> MKKEKIDLFYGALLADIGKVIQRATGERKKHALVGADWFDEIADNQVISDQIRYHMANYQSDKLGNDHLAYITYIADNIASGVDRRQSNEESDEDTSAKIWDTYTNQADIFNVFGAQTDKRYFKPTVLNLKSKPNFASATYEPFSKGDYAAIATRIKNELAEFEFNQVQIDSLLNLFEATLSFVPSSTNTKEIADISLADHSRLTAAFALAIYDYLEDKGRHNYKEDLFTKVSAFYEEEAFLLASFDLSGIQDFIYNINIATNGAAKQLKARSLYLDFMSEYIADSLLDKLGLNRANMLYVGGGHAYF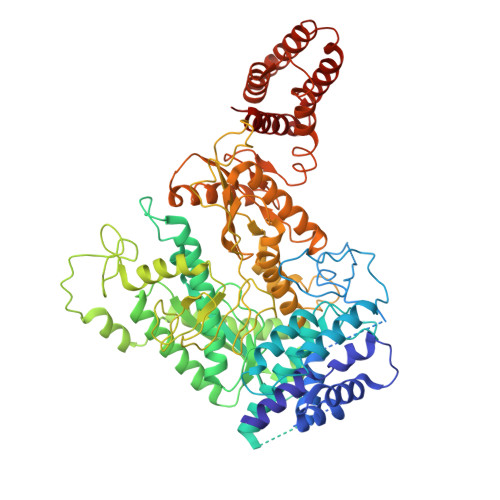VLANTEKTVETLVQFEKDFNQFLLANFQTRLYVAFGWGSFAAKDIMSELNSPESYRQVYQKASRMISKKKISRYDYQTLMLLNRGGKSSERECEICHSVENLVSYHDQKVCDICRGLYQFSKEIAHDHFIITENEGLPIGPNACLKGVAFEKLSQEAFSRVYVKNDYKAGTVKATHVFVGDYQCDEIYNYAALSKNENGLGIKRLAVVRLDVDDLGAAFMAGFSQQGNGQYSTLSRSATFSRSMSLFFKVYINQFASDKKLSIIYAGGDDVFAIGSWQDIIAFTVELRENFIKWTNGKLTLSAGIGLFADKTPISLMAHQTGELEEAAKGNEKDSISLFSSDYTFKFDRFITNVYDDKLEQIRYFFNHQDERGKNFIYKLIELLRNHDRMNMARLAYYLTRLEELTRETDRDKFKTFKNLFYSWYTNKNDKDRKEAELALLLYIYEIRKD> GSHMLEMRIGHGFDVHAFGGEGPIIIGGVRIPYEKGLLAHSDGDVALHALTDALLGAAALGDIGKLFPDTDPAFKGADSRELLREA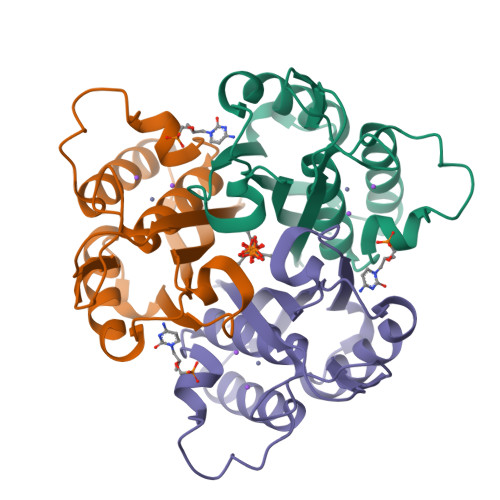WRRIQAKGYTLGNVDVTIIAQAPKMLPHIPQMRVFIAEDLGCHMDDVNVKATTTEKLGFTGRGEGIACEAVALLIKATK> SKYGLQDSDEEDDQLNSAEAKKLKTAPVPPQGKQPPLQQATLPGKVTPPPQSPAVDQLDRVMELDSDMADITQDQDLDSVAEEQDISEEQEPLSASSHIASSLGINPHALQVMKASLLLEEEDGEIMSRFSSFPSSMDPYPDVRSPRLFPSSHAKRPSSIGLLQSKFSAPSMSRLSETVQGSHSPKIHPAAPWSVPAPLAPSFIMPGPAPDTHLRTVGTRRQQELVPLEKSVTHGRGTLMIDMGLFMGRSFRVGWGPNWTLVHNGDKLSERLNAEEDRDMDTIDYGFLPKPTSAKSLTESPFKVHVEKLSLEQKTKDLQSYLLPLEIELKNSTVDKSGPCPHFRPNPGVTAIHDY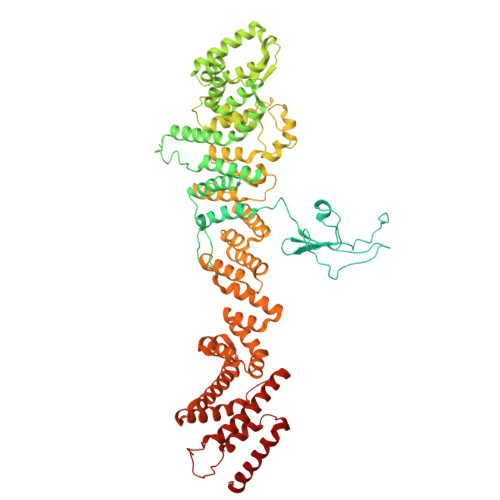AGWVRNFSSEAAEVEAVVKQWGLTWTLCESLWGQLKELEASLDEPNEYVKNLERRKAFSHWLAQTAQERIEEEVSLYGPERHIEAVFSYLTGGRISDACRLAQKSGDHRLSLLLSQMVGSQEVRDLITLQLVDWNKLQVDHYIQEERLRVFCLLSGTPVWRSSDNRSINVCSQLDWKRTLGIHLWYMLPPTATVAQALHMYEQAFQEQEGGEPYACYPLPPYLEDCGFSFGDDPSAKFISLQRDVCVHLLKLYSERQYDLCQLLDPSSATPDPLDYRLSWHMWMVLQALNYTHLSGHRQGMLHASYAAQLENVGLWEWAIFVLLHIQDPHVREAAVRELLNRHCVVHDSPESLAKENFLIQRLCLPAQWIHKAKAVRSRRDGDKHKEALYLLKSHQWNQCHKLVTRHLAADAVINENYRYLRGFLGELARPEHCKHIQDWETAGKVYLDYISVIEMLNQIRQDECSGGELEKLHTKVMSLCKWVELIQCYSAKGRLAQSEMAKRVANILRVVLSLQQPPESMSDSSSEPRVPLRLLAPHIGRLPMPEDYALEELRGLTQSYLRELICGS> SKKHTGYVGLKNQGATCYMNSLLQTLFFTNQLRKAVYMMPTEGDDSSKSVPLALQRVFYELQHSDKPVGTKKLTKSFGWETLDSFMQHDVQELCRVLLD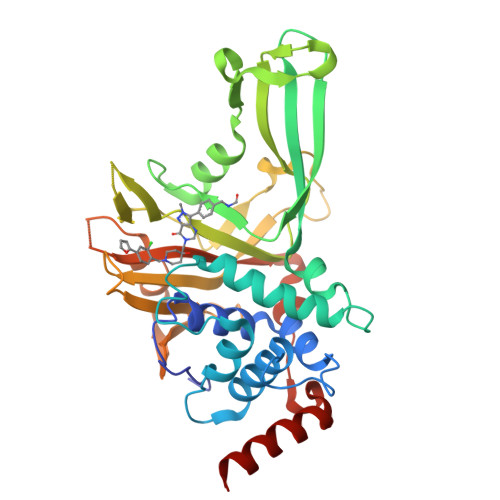NVENKMKGTCVEGTIPKLFRGKMVSYIQCKEVDYRSDRREDYYDIQLSIKGKKNIFESFVDYVAVEQLDGDNKYDAGEHGLQEAEKGVKFLTLPPVLHLQLMRFHYDPQTDQNIKINDRFEFPEQLPLDEFLQKTDPKDPANYILHAVLVHSGDNHGGHYVVYLNPKGDGKWCKFDDDVVSRCTKEEAIEHNYGGHDDDLSVRHCTNAYMLVYIRESKLSEVLQAVTDHDIPQQLVERLQEEKRIEAQK>[2x]MQRCDWVSQDPLYIAYHDNEWGVPETDSRKLFEMICLEGQQAG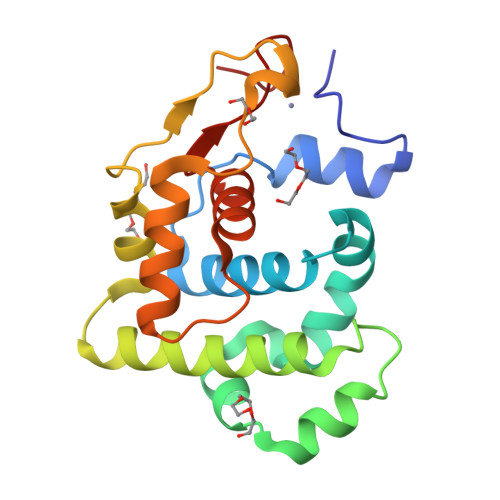LSWITVLKKRENYRACFHQFDPIRIAAMQEEDVERLLQNTGIIRHRGKIQAIISNARAWLAMEQNGESFADFVWSFVDGQPQITQAASLDKIPTSTPASDALAKALKKRGFKFVGTTICYSFMQACGLVNDHITGCFCHP>MLKGKVAVVTGSTSGIGL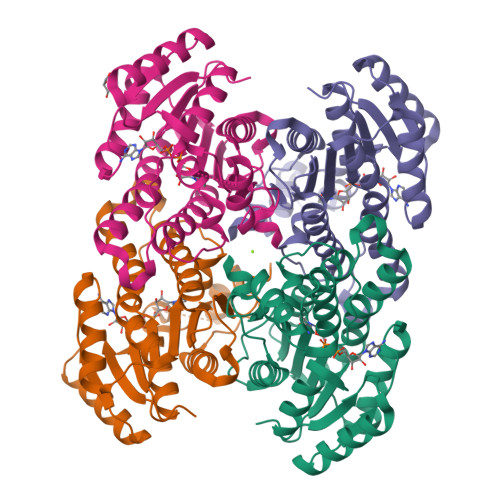GIATALAAQGADIVLNGFGDAAEIEKVRAGLAAQHGVKVLYDGADLSKGEAVRGLVDNAVRQMGRIDILVNNAGIQHTALIEDFPTEKWDAILALNLSAVFHGTAAALPHMKKQGFGRIINIASAHGLVASANKSAYVAAKHGVVGFTKVTALETAGQGITANAICPGWVRTPLVEKQISALAEKNGVDQETAARELLSEKQPSLQFVTPEQLGGTAVFLASDAAAQITGTTVSVDGGWTAR[4x]> SQLTPRRPYLLRAFYEWLLDNQLTPHLVVDVTLPGVQVPM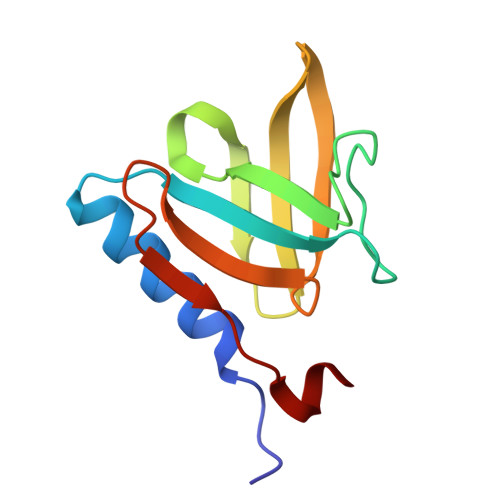EYARDGQIVLNIAPRAVGNLELANDEVRFNARFGGIPRQVSVPLAAVLAIYARENGAGTMFEPEAAYD>[3x]EVYGIIAMQAAYRDYDSGDAKQDDNLGGMQLNNESRIGFRGKKQFANFEPTFIWQIEGGYVDPSFGGEGAGLGERDTFVGF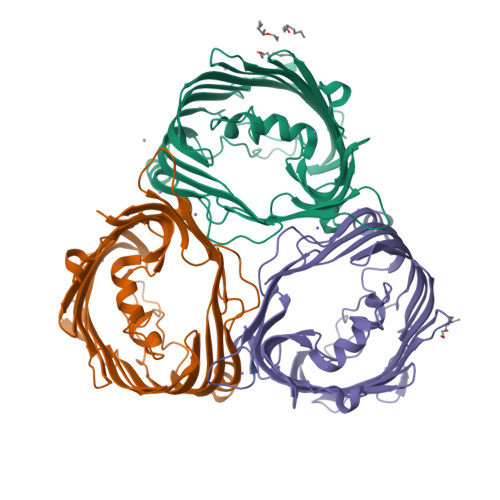ESASWGQVRLGRVLTPMYELVDWPASNPGLGDVYDWGGAIGGAKYQDRQSNTIRWDSPMYADKFSIDAAVGAGDKAGLGAGDDYWGGIAAHYKLGPLQLDAAYEGNRNIEAEGQTWENNTYLVGVQGWFENGISFFAQYKYMEADASNGVNEKQDAMSAGLMYTTGDWQYKLGYAANFDLERDGKTLSNTSDDVVSAQIMYFVDPSAVLYARARMNDFNEGLDGLDDAARWTSGTNGDYNEYSVGVEYYF> MEDINFASLAPRHGSRPFMGTWNEIGTSQLNGGAFSWSSLWSGIKNFGSSIKSFGNKAWNSNTGQMLRDKLKDQNFQQKVVDGLASGINGVVDIANQALQNQINQRLENSRQPPVALKQRPTPEPEEVEVEEKLPPLETAPPLPSKGEKRPRPELEETLVVESREPPSYEQALKEGASYPMTRPIGSMARPVYGKEKTPVTLELPPPAPTVPPMP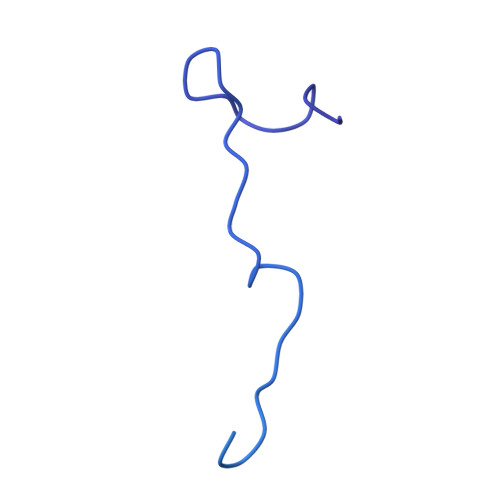TPTLGTNVPRLAAPTVAVATPARRVRGANWQSTLNSIVGLGVKSLKRRRCY>MEKRMSTQQRAAGNACPTAAFSFDPARLAQRRRWAGAFAALCGLALSPSALLAEEHSQHQDHAVELAPSVVTGVAQSSPLTIVTNPKEPRQPVPASDGADYLKTIPGFAVIRNGGSNGDPVLRGMFGSRLNILTNGGMMLGACPNRHDAPTSYISPETYDKLTVIKGPQTVLWGPGASAGTILFEREPERFGELGSRVNASLLAGSNGRFDKVLDAAAGNRLGYL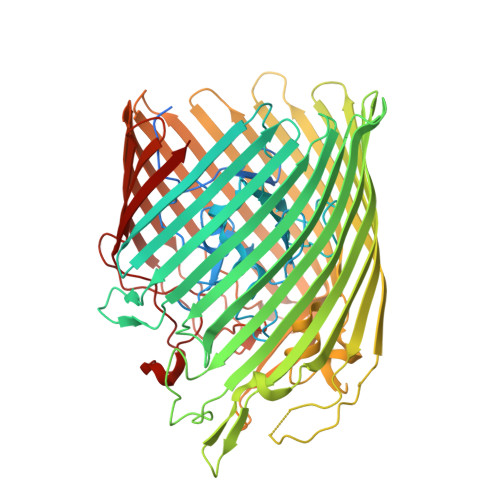RFTGNHAQSDDYEDGAGNTVPSRWKKWNGDVAVGWTPDEDTLIELTAGKGDGEARYAGRGMDGSQFKRESLGLRFVKSNVSDVLEKVEAQVYYNYADHIMDNFRLRTPDPSSMMPMPMASQVDRRTLGGRLAATWRWDDFKLVTGVDAMRNEHRARGSKYDMMTDYYTDADQFPWSKDAVFHNYGAFGELTWFAAERDRLIGGLRLDRASVKDYRQTLKSGHMGHAMANPTANDTRADTLPSGFVRYEHDLADSPTTLYAGLGHAERFPDYWELFSPKRGPNGSVNAFDKIKPEKTTQLDFGLQYNGDKLQAWASGYVGVVQDFILFSYREGMMGSSTQATNVDARIMGGELGASYQLTGNWKTDASLAYAWGKNSSDDRALPQIPPLEARFGLTYEEGDWSAGSLWRVVAPQNRIARDQGNVVGKDFDKSAGFGVFSLNGAYRVTRNVKLSAGVDNLFDKDYTEHLNKAGDAGFGFSANETVPEPGRTFWTKVDFSF[2x]Substrate selection occurs in the cytoplasm and inner membrane, mediated by the export gate subcomplex (EscRSTUV in EPEC, and FliPQR, FlhB, FlhA in flagella) and the cytoplasmic ATPase complex (ATPase EscN, peripheral stalk EscL, and central stalk EscO; flagellar FliI, FliH and FliJ, respectively). The T3SS ATPase homologues are made distinct by their homohexameric construction, a presumed ancestral precursor to the heterohexameric rotary F1/V1-ATPases. The ATPase has been proposed to specifically enhance PMF-induced secretion efficiency, as well as to play a role in effector targeting, release from chaperones and unfolding prior to secretion. Each EscN monomer displays three sub-domains: the N-terminal oligomerization domain (residues 1–102), a cluster of curved β-sheets; the ATPase domain (103–372), made up of a central Rossmann fold with seven parallel β-strands flanked by four α-helices on one side and three on the other; and the C-terminal domain (373–446), made up of four helices lining the central pore.

The EscN-EscO complex was subjected to single-particle cryo-EM, with 3D classification resulting in two primary classes that refined to high resolution. Class 1 (58,000 particles, 3.34 Å) reveals a homohexameric EscN pore lacking visible EscO density, while class 2 (55,000 particles, 3.29 Å) looks similar but with additional α-helical density for approximately half of a single EscO molecule resolved. The final refined model spans residues 35–446 for all chains, excepting unresolved loop 323–329 on chain NF. The EscN hexameric structure shows marked asymmetry, with a prominent cleft between chains NA and NF. The N-terminal domain is largely static between subunits, with approximate C6 symmetry around the pore axis. Aligning each EscN chain by the N-terminal domain highlights a key pivot point between the N- and ATPase domains, with the ATPase and C-terminal domains essentially moving as a rigid body from subunit to subunit. Subunit NF, the most dynamic monomer with the least resolved density, is tilted back nearly 30° relative to the most inward angled subunit ND, indicating impressive motion at this pivot point. In four of the six EscN inter-subunit active sites, the Mg2+ADP-AlF3 transition state analogue was clearly visible; the resolution was insufficient to differentiate between AlF3 and AlF4, so AlF3 was used as the more abundant species at pH 7.530. The EscN active site location at the subunit interface and key motifs are conserved with the latter, including the P-loop (residues 179–185), catalytic glutamate (Glu206), and arginine finger (Arg366). The structure presented here shows that EscN can adopt similar C-terminal domain conformations; the lever is closed in nucleotide-bound sites T through D′, and open in nucleotide-free sites E and E′.

>GSHMISEHDSVLEKYPRIQKVLNSTVPALSLNSSTRYEGKIINIGGTIIKARLPKARIGAFYKIEPSQRLAEVIAIDEDEVFLLPFEHVSGMYCGQWLSYQGDEFKIRVGDALLGRLIDGIGRPMESNIVAPYLPFERSLYAEPPDPLLRQVIDQPFILGVRAIDGLLTCGIGQRIGIFAGSGVGKSTLLGMICNGASADIIVLALIGERGREVNEFLALLPQSTLSKCVLVVTTSDRPALERMKAAFTATTIAEYFRDQGKNVLLMMDSVTRYARAARDVGLASGEPDVRGGFPPSVFSSLPKLLERAGPAPKGSITAIYTVLLESDNVNDPIGDEVRSILDGHIVLTRELAEENHFPAIDIGLSASRVMHNVVTSEHLRAAAECKKLIATYKNVELLIRIGEYTMGQDPEADKAIKNRKLIQNFIQQSTKDISSYEKTIESLFKVVA[6x]>MGAIESRKLLASETPVGQFIPYSHHVTDTIISTKNAEYLSVWKIDGRSHQSASEADVFQWIRELNNTLRGISSANLSLWTHIVRRRVYEYPDAEFDNVFCRQLDEKYRESFTGYNLMVNDLYLTVVYRPVSDKVLSFFAKRERETPDQKKHRQESCIKALEDINRTLGQSFKRYGAELLSVYEKGGHAFSAPLEFLARLVNGEHIPMPICRDRFSDYMAVNRPMFSKWGEVGELRSLTGLRRFGMLEIREYDDATEPGQLNVLLESDYEFVLTHSFSVLSRPAAKEYLQRHQKNLIDARDVATDQIEEIDEALNQLISGHFVMGEHHCTLTVYGETVQQVRDNLAHASAAMLDVAVLPKPVDLALEAGYWAQLPANWQWRPRPAPITSLNFLSFSPFHNFMSGKPTGNPWGPAVTILKTVSGTPLYFNFHASKEEEDATDKRLLGNTMLIGQSSSGKTVLLGFLLAQAQKFKPTIVAFDKDRGMEISIRAMGGRYLPLKTGEPSGFNPFQLPPTHANLIFLKQFVKKLAAAGGEVTHRDEEEIDQAITAMMSDSIDKSLRRLSLLLQFLPNPRSDDMDARPTVHARLVKWCEGGDYGWLFDNPTDALDLSTHQIYGFDITEFLDNPEARTPVMMYLLYRTESMIDGRRFMYVFDEFWKPLQDEYFEDLAKNKQKTIRKQNGIFVFATQEPSDALESNIAKTLIQQCATYIFLANPKADYEDYTQGFKLTDSEFELVRGLGEFSRRFLIKQGDQSALAEMNLGKFRTIVDGETVERDFDDELLVLSGTPDNAEIAESIIAEVGDDPAVWLPIFLDRVKAERSDVGSGSGSAVDMFIKIGDVKGESKDKTHAEEIDVLAWSWGMSQSGSMHMGGGGGAGKVNVQDLSFTKYIDKSTPNLMMACSSGKHYPQAKLTIRKAGGENQVEYLIITLKEVLVSSVSTGGSGGEDRLTENVTLNFAQVQVDYQPQKADGAKDGGPVKYGWNIRQNVQA[6x]

In Gram-negative bacteria, conjugation is mediated by a large transport apparatus—the conjugative type IV secretion system (T4SS)—produced by the donor cell and embedded in both its outer and inner membranes. The T4SS also elaborates a long extracellular filament—the conjugative pilus—that is essential for DNA transfer. Here we present a single-particle cryo-EM structure of a T4SS complex from the R388 plasmid that comprises all four sub-complexes: OMCC, stalk, arches and IMC. Three ATPases, VirB4 (also known as TrwK), VirB11 (also known as TrwD) and VirD4, power the system.

We first solved the structure of VirB4 in its unbound form (VirB4unbound) and fitted and rebuilt the structure within the IMC density. NSEM provides a view of a double-barrelled IMC made of two side-by-side trimers of dimers (the barrels) of the AAA+ VirB4 ATPase, whereas cryo-ET shows a central hexamer of dimers of the same protein. Of note, a minority of the 2D classes in our cryo-EM data set displayed the typical side-views of the double-barrelled architecture observed in the NSEM structure, indicating the presence of a small number of double-barrelled particles.>YGAGQIQVLEGLEAVRKRPGMYIGSTSERGLHHLVWEIVDNSIDEALAGYANQIEVVIEKDNWIKVTDNGRGIPVDIQEKMGRPAVEVILTSSVVNALSQDLEVYVHRNETIYHQAYKKGVPQFDLKEVGTTDKTGTVIRFKADGE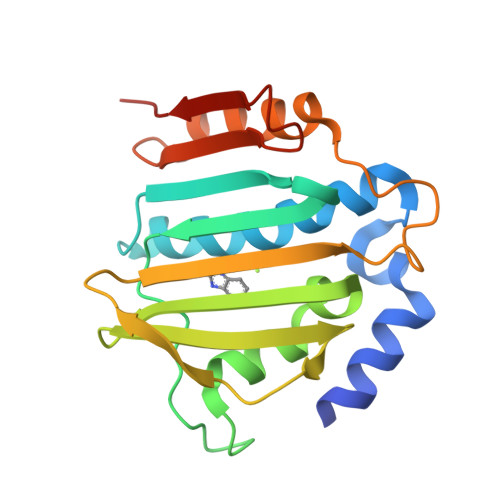IFTETTVYNYETLQQRIRELAFLNKGIQITLRDERDEENVREDSYHYEGGI[2x]>[6x]MYNDDYIEEASFLNGSDVVILIDGVEELYMEEIKADFEQDEQSIKLLGCQNEISRVGTTKGSFSLNGYKTDSKFAKLGFRSFEIIYNLSNSETLGYESIRLKNCRLKKLPLINSKAGEIVKIEVEGSFRGYDLLNEL;>[6x]MINIDRRRKDIIRTININPTNITITSIKKTEIDGAFEETETEIKCVVRIFNEKTAEKQISSEKQGTFSSIRTYGMLVSNDVILEVNSRDSLEFECIYGRMKIVNIYPQIVKGELCGYQCSLERID;>MRAGIRKALIDNIKELKGCYEPNVPNKDTKKPYMVVVQGQDNDHGETIGFERSIEVWIYEGRTTFKKLDKLTKQVVEVLDMNTIVDESENEAFTCIYKGTSENDIVVEEWDAIARGIRFSVIALEDKEDTTNDRWVEALSRHTKDLLEIESYKDNWKKNFIAPCALWRTTHIENKRINYHLIEITKTMKCHVVSKNKDEIVKLLETLETSLIIDKRVRLREDKNMYLTLVSVVEDRESDMFTTGQLTAVFKMIGKIKREGPTMDKIYGNGNLK[6x];>[12x]MTPARDLIEKLRLLLNDKDKKSFTDEELNLFLEEADCIYCAASQGWILKSLQYENTVGEMYEYKVGQETYKSSSIKDLVSVAYQNADKFKDMCTNKKEKGSFMLGISTEFEI;>MATGTWNEKERKEIPGFYNRFKTQAEKSTNTGLKGRLAMPIRANWGDVGKVVTIKNDLRQLKNLFGDDMNYSAFKLGKLALLGNVKELLLYRLVDGNQKKGTLTLKDTTENSAKDVIKLETKYPTARNFNVTIKSNLVDSDKKDFIFFENTKQLFSSSIKGTIDEIVLEINSNLDNEYVIATKVADSDTILANVVNQALEGGNDGCTSITNESYLKALEEFERYSFDSFVLDGVADEALQETTKAWVAKNKELGKDILLFLGGKTEDNIKQINDKSKSFNDENIVNVGSSAYYENIKYTPSEVAVYIAALSVSKGITGSICNAKTIFEEVEPRLSQSEVKECLKSGTLVLDFDDGDVIIVDDVNTFKKYVDDKNEAMGYISNIMFINTINKDTSLKRKEFVGKIFNDATGQTTVICALKKYFEELMSQGIISEFNVDIDTELQATAKADEFYWKWDAVKVDVMKKIYGTGYLG[6x];>MGIISYVKKLFKRPAGEIMRMSSGNIGVYKLDDSRVDYELARELYQNKNANYKLGSSFVRPIVNSTTGFMGVPHFQIEDEEAQYILDEFVLDNTSKMLKTHTDSLKQGDCYIWITREERENPLYPDKKVRLIYNFISPEEVKEIILDPTTKEPIAYILESQNEWTDLGENKRKAKVKQIITAESRFVEVEGDKIEGLEEGETPNVWGFIPIIHFKNEADETLKYGQSDIEPIEPLLKAYHDVMLHALKGSKMHSTPKLKLKLTDVASFLAHNFGVEDPVKFAKEGGKINLDGHEILFLNKDEEAEFVEVKSAIGDAKELLKLLFYCIVDVSETPEFIFGVHTPSALASVKEQMPIMVNKIRRKREQFTNSWQLLARMVLIMSSNSSGMKYSSYDVTIGWDEVNPRDDKELAETLEKVCCALDKALEGGFISEESTVNFLAQYIDTMSNYISDDGEREGEREKIIKTKMLKYRLDDSQGLNDESNEIEKEINKIKDNNGNG[12x]

Here, we reveal the extended and contracted atomic structures of an intact contractile-tailed phage (φCD508) that binds to and penetrates the protective S-layer of the Gram-positive human pathogen Clostridioides difficile. The virion can be divided into five distinct regions: the head, neck, tail, baseplate, and needle. Structures of purified φCD508 virions in both extended and contracted conformations were determined by single-particle EM of frozen-hydrated samples; the resolution ranged from 2.6 to 4.0 Å for the extended phage, and 2.9 to 4.2 Å for the contracted form.

The overall RMSD between all proteins of the neck in the extended state compared with the contracted state is 0.34 Å, indicating that no large conformational change occurs in this region during phage contraction. After contraction and genome release, the neck-proximal tail sheath protein (gp55) remains attached to the tail terminator gp53 via its C-terminal insertion domain. The neck-proximal sheath protein rotates to accommodate the contraction-induced movements of the other sheath proteins in the tail below, pivoting around Gly260 in the gp53 C-terminal linker. The terminal sheath ring proximal to the neck proteins still maintains some contact with the tail tube. This reduced rotation is limited to the proximal layer, with the next layer below fully dissociating from the tail tube, similar to the arrangement observed for the main body of the contracted tail reconstruction.>[4x]GSNNSETPAPGPDSLLALAFPSDPQVSPDGKQVAFVLAQISEEDPAKPDKDFARPRYRSGLWLSEGGAARPLTHAETGRGDSAPRWSPDGQNLAFVRSAGEVKAALMLLPLKGGEARRVTHFKNGVSGPQWSPDGRFIAFTTTADTEDKRDERGEARVLTRPVYRANGADWLPERPAALWLYDVEADKLREWYAPEIGIGALSWWPDSRGVLIVQSEDEWQASQWRQDVYDLPLPTADAPAAPQKLLDWNSAAHGLAPHPDGQRFALIGRPAGKGNTEHAHLYLIENGQHRRLDTGHDHPVGDAVGGDCHVGAFPEGPRWLDGDTLLFSSTVRGSVGLFTAHIGGGVKAYDHDPQ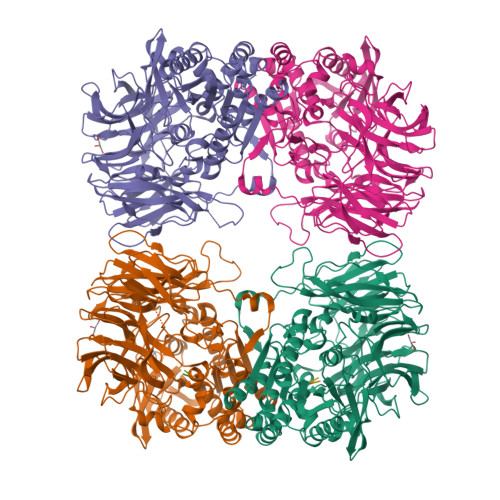GVISAFTANEHGVALIRESATRFPEVELNGQRVTDLHARFPFPVREPQRVTFETELGEGEGWVLLPEGEQKVPALLNIHGGPHTDYGHGFTHEFQLMAARGYGVCYSNPRGSVGYGQAWVDAIYGRWGTVDADDLLNFFDRCLEAVPRLDAAKTAVMGGAYGGFMTNWITGHTTRFQAAITDRCISNLISFGGTSDIGLRFWDDELGLDFSRRADALKLWDLSPLQYVENVKTPTLIVHSVLDHRCPVEQAEQWYAALHKHQVPVRFVRFPEENHELSRSGRPDRRLTRLNEYFAWLERWL;>MAA[2x]>[3x]MAHHHHHHMERTYIMVKPDGVQRGLIGEILKRFEMKGLKLIAAKFEHPTMDVVAQH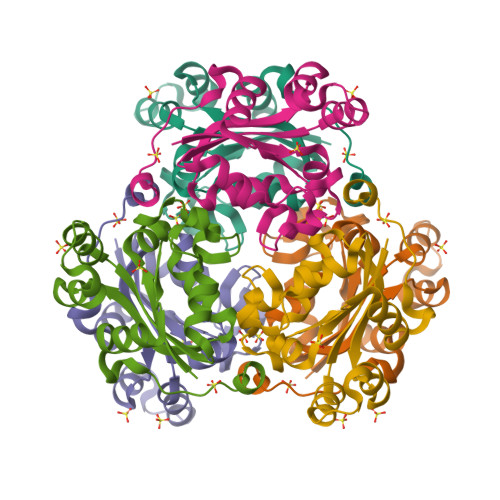YCEHKDKPFFKDLCDFISHGPVFCMIWEGPEAIKIGRNLVGLTSPVESAAGTIRGDFGVVKNFNIVHASSSAEDAARECALWFTPEQLVTWERSVGGWIY>GMEQQHPTIHTLKIETEFFKAVKERRKTFEIRKNDRNFQVGDIL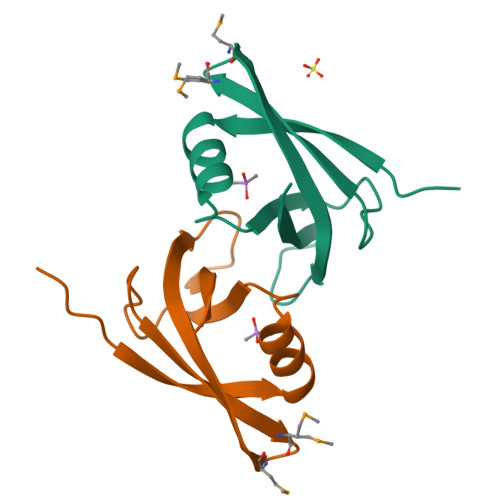ILEEYMNGMYLDDECEAEVIYITDYAQREGYVVLGIELH[2x]>[3x]MISNNAPAKMVLNSVLTGYTLAYIQHSIYSDYDVIGRSFWLKEGSNVTRRDFTGIDTFSVTINNLKPTTTYEVQGAFYDSIIDSELLNAQIGINLSDKQTFKMKSAPRITGARCESEPVDVGVGAPIVYIDTTGEADYCTIELKDNSNANNPWVKYYVGALMPTIMFGGVPIGSYKVRISGQISLPDGVTIDSSGYYEYPNVFEVRYNFVPPAAPINIVFKAARIADGKERYDLRVQWDWNRGAGANVREFVLSYIDSAEFVRTGWTKAQKINVGAAQSATIISFPWKVEHKFKVSSIAWGPDAQDVTDSAVQTFILNESTPLDNSFVNETGIEVNYAYIKGKIKDGSTWKQTFLIDAATGAINIGLLDAEGKAPISFDPVKKIVNVDGSVITKTINAANFVMTNLTGQDNPAIYTQGKTWGDTKSGIWMGMDNVTAKPKLDIGNATQYIRYDGNILRISSEVVIGTPNGDIDIQTGIQGKQTVFIYIIGTSLPAKPTSPAYPPSGWSKTPPNRTSNTQNIYCSTGTLDPVTNQLVSGTSWSDVVQWSGTEGVDGRPGATGQRGPGMYSLAIANLTAWNDSQANSFFTSNFGSGPVKYDVLTEYKSGAPGTAFTRQWNGSAWTSPAMVLHGDMIVNGTVTASKIVANNAFLSQIGVNIIYDRAAALSSNPEGSYKMKIDLQNGYIHIR

In siphophage T5, the unique RBP is located at the extremity of a central fiber. FhuA, an outer membrane E. coli iron-ferrichrome transporter, is the bacterial receptor recognized by T5 (25). We present the structures of T5 tail tip, determined by cryo–electron microscopy before and after interaction with its E. coli receptor, FhuA, reconstituted into nanodisc. These structures bring out the important conformational changes undergone by T5 tail tip upon infection, which include bending of T5 central fiber on the side of the tail tip, tail anchoring to the membrane, tail tube opening, and formation of a transmembrane channel.

(D) Cryo-EM structure of the central fiber at 4.2-Å resolution. BHPpb3 C-terminal ~210 residues and pb4 N-terminal ~350 residues were modeled de novo. The proximal region of the central fiber is made of three strings of five consecutive FNIIIs, two at BHPpb3 C terminus and three at pb4 N terminus. After a hinge region, the three pb4 monomers merge to form a 110-Å-long β helix spike, formed of a 24 β strand longitudinal mixed β sheet prism. The spike is decorated with two small globular domains inserted between β strands 15 and 16 of each pb4 subunit and which are connected by relatively long linkers. These domains are not visible in the central fiber map, probably because of the degrees of freedom offered by the linkers. Here, however, pb4 does not have a direct role in perforation or host recognition. The central fiber ends with RBPpb5, but this part of the map is poorly resolved and did not allow building an atomic model of this protein. This 310-Å-long central fiber bears two hinges, one between pb4 last FNIII and the spike and the other at the spike-RBPpb5 interface: It introduces some controlled flexibility to this otherwise rigid assembly and may ease RBPpb5 exploring space and encountering its bacterial receptor.> GSMIRSTLSSWREYLTPITHKSTFLTTGQITPEEFVQAGDYLAHMFPTWKWNEESSDISYRDFLPKNKQFLIIRKVPADKRAEQAVEVEGPDVIMKGFAEDGDEDDVLEYIGSETEHVQSTPAGGTKDSSIDDIDELIQDMEIKEEDENDDTEEFNAKGGLAKDMAQERYYDLYIAYSTSYRVPKMYIVGFNSNGSPLSPEQMFEDISADYRTKTATIEKLPFYKNSVLSVSIHPCKHANVMKILLDKVRV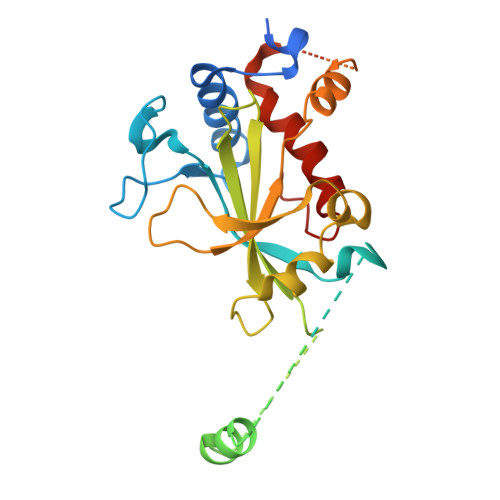VRQRRRKELQEEQELDGVGDWEDLQDDIDDSLRVDQYLIVFLKFITSVTPSIQHDYTMEGW>MSIPVTEFRQFSEQQPAFRVLKPWWDVFTDYLSVAMLMIGVFGCTLQVMQDKIICLPKRVQPAQNHSSVPNVSQAVISTTPLPPPKPSPTNPATVEMKGLKTDLDLQQYSFINQMCYERALHWYAKYFPYLVLIHTLVFMLCSNFWFKFPGSSSKIEHFISILGKCFDSPWTTRALSEVSGEDSEEKDNRKNNMNRSGTIQSGPEGNLVRSQSLKSIPEKFVVDKSAAGALDKKEGEQAKALFEKVKKFRLHVEEGDILYAMYVRQTVLKVIKFLIIIAYNSALVSKVQFTVDCNVDIQDMTGYKNFSCNHTMAHLFSKLSFCYLCFVSIYGLTCLYTLYWLFYRSLREYSFEYVRQETGIDDIPDVKNDFAFMLHMIDQYDPLYSKRFAVFLSEVSENKLKQLNLNNEWTPDKLRQKLQTNAHNRLELPLIMLSGLPDTVFEITELQSLKLEIIKNVMIPATIAQLDNLQELCLHQCSVKIHSAALSFLKENLKVLSVKFDDMRELPPWMYGLRNLEELYLVGSLSHDISKNVTLESLRDLKSLKILSIKSNVSKIPQAVVDVSSHLQKMCVHNDGTKLVMLNNLKKMTNLTELELVHCDLERIPHAVFSLLSLQELDLKENNLKSIEEIVSFQHLRKLTVLKLWYNSIAYIPEHIKKLTSLERLFFSHNKVEVLPSHLFLCNKIRYLDLSYNDIRFIPPEIGVLQSLQYFSITCNKVESLPDELYFCKKLKTLKIGKNSLSVLSPKIGNLLFLSYLDIKGNHFEVLPPELGDCRALKRARLVVEDALFETLPSDVREQMKADALEVLFQ[7x]

Volume-regulated anion channels (VRACs) participate in the cellular response to osmotic swelling. These membrane proteins consist of heteromeric assemblies of LRRC8 subunits, whose compositions determine permeation properties. VRACs are composed of proteins belonging to the conserved LRRC8 family, whose expression is restricted to chordates. This family contains five members in humans, termed LRRC8A–E. All of them share a close sequence relationship and consist of an N-terminal pore domain (PD) followed by a cytoplasmic leucine-rich repeat domain (LRRD). In these assemblies, LRRC8A (or SWELL1) constitutes an obligatory subunit, which is essential for the targeting of channels to the plasma membrane.

We then set out to characterize the full-length protein and collected cryo-EM data for an LRRC8C homomer from three independent preparations. Unexpectedly, the two-dimensional (2D) classes from these datasets showed in all cases a heptameric assembly, which was confirmed by 3D reconstruction. Despite the large size of the combined dataset, the non-symmetrized reconstruction of the full-length protein did not reach high resolution, probably due to the intrinsic mobility of the complex. After application of C7 symmetry, we were able to obtain a structure extending to 4.6 Å for the full-length protein and 4.1 Å for the PD. At low contour, the map displays an envelope for the entire protein, and at higher threshold, where the density of the more mobile LRRDs has largely disappeared, it defines the structure of its membrane-inserted portion. This map allowed a molecular interpretation with subunits consisting of the structure of the PD determined by cryo-EM and the X-ray structure of the LRRD to obtain a symmetric channel with a pore radius of 6 Å at its extracellular constriction. In this assembly, close subunit interactions are restricted to the extracellular part, whereas contacts within the remainder of the protein are scarce. In contrast, there are fewer contacts in the case of LRRC8C homomers, which have formed a larger heptameric assembly. In this case, the LRRDs show increased mobility compared to the A subunits, and we did not find any indication of tight subunit interactions. Similarly, the interaction interface in the PD is reduced and restricted to contacts between the ESDs. In that respect, the larger heptameric assembly of LRRC8C homomers described in this study is noteworthy, as it would allow for a further increase of the pore radius, although there is so far no evidence for the existence of heteromeric channels with larger oligomeric organization in a physiological context.>[2x]MCGVAGWVSFRQDLSHEENILAGMTNSMTCRGPDASGQWLSRHAALGHRRLSIIDLPGG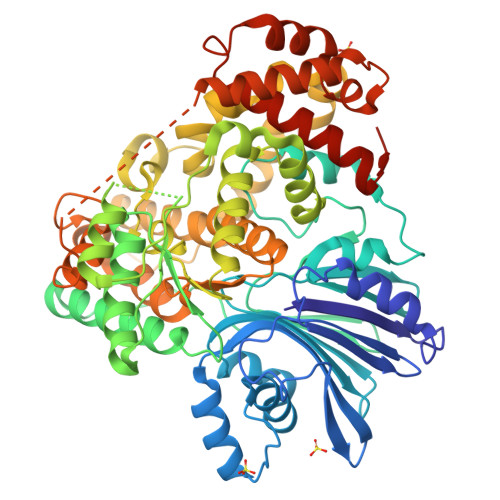TQPMTVDTPGGPVTMSYSGETYNFVELRDELRKRGHTFRTRSDTEVVLRGYLEWGAAIAERMVGMCAIAIWDSRYERLTLIRDRMGTKPMHYYRTKDGLLFGSEPKAILAHPDVKPVVDMEGMRQLFSFFTSSENAVWADMKVMTPGTVIEFDRNGLREHTYWQLSAEEHTDDLDTTVARVRQMVEDNVRHELVADVPLGLLLSGGLDSSALAGIASRHLTAKGERARTFSVDFPGQSENFQPHEMADSADAPYAKEMAAHIGSEHHDIVLDHRRLSDPDLRRSVVAAWDLPWGMGDINGSMYLLFKAVREHVTVALSGEAADEIFAGHVWHQSKAARYGGTFPWHTTWLKRVDCSAYLTGEFNAALDSETYTADRFQEATARVPYLDGEDEEQRMYRRSLHLGLNHFMRVLEDRVDRMAMAVGLETRVPFCDYRLAQYLYNVPWTMQTFDGREKSLLRASVTDVVTPSVVARRKSPYPSTQDTLYVGALQEQVKILLKEPSSPVFDLFDRSKLAEAAELSPQQIAGAPRAAFEKALDLAVWFEIRNPELRYLVPRGSHHHHHH> GSHMMKRLVFISKISGHLSLEEIQRIGKVSIKNNQRDNITGVLLYLQGLFFQILEGENEKVDKLYKKILVDDRHTNILCLKTEYDITDRMFPNWAMKTINLNENSELMIQPIKSLLQTITQSHRVLEKYMPARVIYLINQGINPLTVEPQLVEKIIFFSDILAFSTLTEKLPVNEVVILVNRYFSICTRIISAYGGEVTKFIGDCVMASFTKEQGDAAIRTSLDII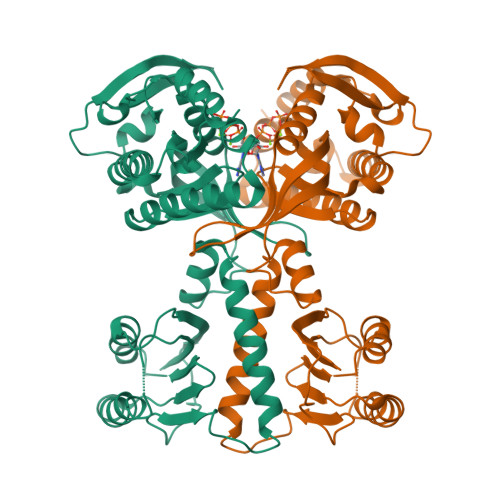SELKQLRHHVEATNPLHLLYTGIGLSYGHVIEGNMGSSLKMDHTLLGDAVNVAARLEALTRQLPYALAFTAGVKKCCQAQWTFINLGAHQVKGKQEAIEVYTVNEAQKYYDTLQITQLIRQTLENDK> MDNPCLKGPPVPKNAAECCVTPFLVEPSAFMTCHSKWIGQTKRQMAMEGIPRGCCVAECVMNSTSLYSNGKIDREALTKLYLDSTKSMAPEWNKITLDAIDGCFKMADSIKDEIEAGAKLTPAFEGEQ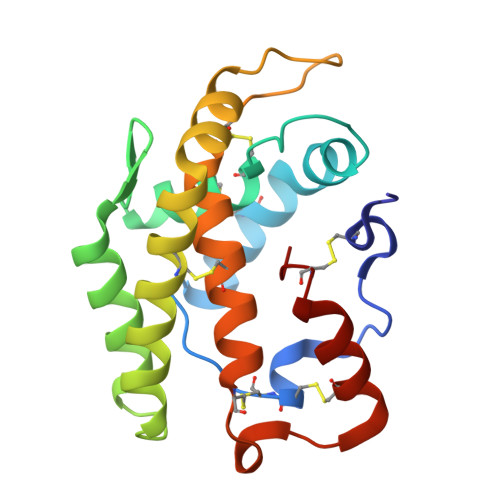ICHPISGTILACMGMTLFAECPAKLFTVNDDCNKLKSYHSKCPFL>[2x]MTVLILTSEEDVTADMVVVHLNASGVPVVRLDPADLTDSVALSGEFAHGSFRGHLSSGGRLVSIGGLRSVWVRRPGGAATRAAEPSAWLTEEAGQALYGMLRGSGARWMNQPDAAHRARYKPWQLRLAQRCGLPVPATLI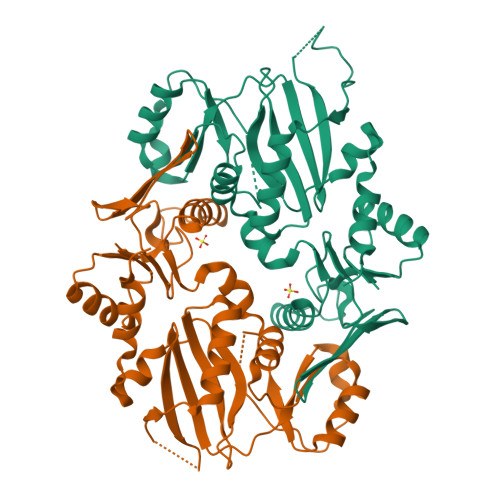TTFPRAAREFAERYPDLVVKPVSGAHPQDPPLAVPTSRVPPEADFSAVAHGPTLLQRRVAKRADIRLTAVGEELLAARKTALASLDPDEVDVRFAGSGEPWRPAEVPPRVAEGVRAYLRAAGLAYGALDFAEDGDGTWWFLECNQSGQFGFVEVDTGQPIARTIAEWLARPGAADAVEPGGPDAAAVGAAALEHHHHHH>[2x]HHHHHHFNLPPGNYKKPKLLYCSNGGHFLRILPDGTVDGTRDRSDQHIQLQLSAESVGEVYIKSTETGQYLAMDTDGLLYGSQTPNEECLFLERLEENHYN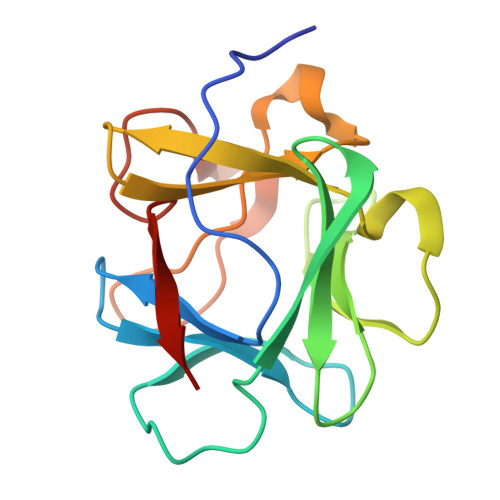TYISKKHAEKNWFVGLKKNGSCKRGPRTHYGQKAILWLPLPVSSD> GPTYVQA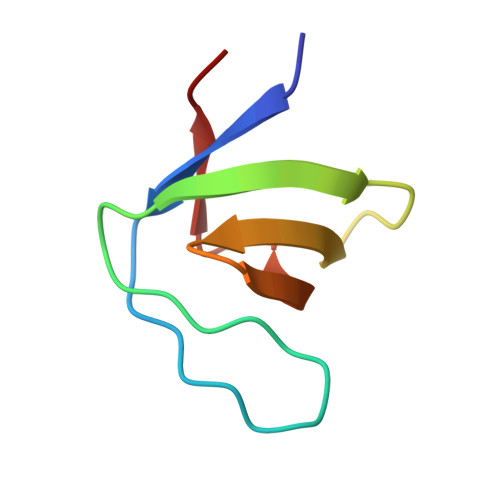LFDFDPQEDGELGFRRGDFIHVMDNSDPNWWKGACHGQTGMFPRNYVTAVN> MDNSNGIHYIELTPNPIRFDAVSQLTNVFFDDSNKQIFAVRSGGATGVVVKGPGSPDDVVISFCMSDRGGAIRSIKFSPDNQILAVQRKENSVEFICFQGDQPLLQDIITHQVKTLIHGFVWVHNREVALISNTGVEVYTVVPEKRQVRSVKSLSIGIKWFAWCCDANVALLCTSEGNSLIPVLVKQKVITKLPKVDLGNPSRDVQESKVTLGQVYGVLAVLILQSNSTTGLMEVEVHLLNGPGLAPRKCHVLRLSLLGRFAINTVDNLIVVHHQASGTSLLFDISLPGEVINEITYHTPITPGRSIKPFGLKLPSLSPDGQILQCELYSTHWVLFQPNIVIDAKLGCMWFLNLCIEPLCQLISDRIRLTEFLLQRSNGKQMLLKVIGQLVDDQYKGTLLPVLETIFSRINKIYASWVQLELQNQTAQPSNVKTTTLKQSTPPIVLIEQLDMVQIFQRIARRPYTESILMLYLQSLNKFNIAAQEELSKMIISELISNRSFDTLRRLVSYSMLLESKSVACFLLSHSNVDTAISQVAIDMLGRIEAHEIIIEVMLGQGKVIDALRLAKNSMGLEKVPARKFLEAAHKTKDDLIFHSVYRFFQMRNLKLYETLSFPKAEQCTEFIQHYNNTFPADNPTRQPVS;> MAKLLQRVEITLRSFYIFNSTFGQVEGEEHKKVLFYHPNDIELNTKIKDVGLSEAIIRFTGTFTSEDDCQALHTQKTTQLFYQPEPGYWLVLVLNVPKEVRLKEGVEVADYRGAEISDRIYRAILRQCYQMFRFQNGCFSSCGSEEPNPDKRRELLCQKLLQFYDQHLTNLRDPAQCDIIDMLHSIQYLPLDKTLFLRAQNFGTLCETFPDIKESIMLYQEQVLCGGKLSPEDLHCVHSYV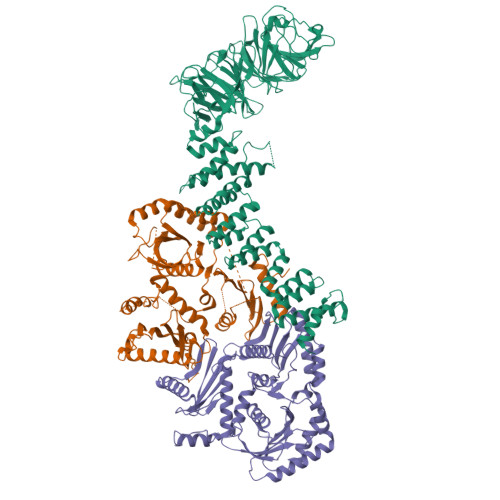VQHVLKVEASSSTIAVSPSLKRSISECQVGGFVRSRQKVAGDEHDAVNEEDHPMKVYVTLDKEAKPYYLLIYRALHITLCLFLNADQVAPKQDLYDDLHAYMAPQLTSLARDISSELTKEAVGAAGQDNSSGNSETAPKYLFINEQSLQHHTNFQRHLPQGLPRNVLSIIADLANGSGKAEMESAPAEEVQVKTTNDYWIVKRRCNYRQYYVILCNSKATLLDVTQEARRIFEQELTDDVFFDK;> HHHHHHHHHHENLYFQGGGSMEVEQTSVRSDTNSTCEYLDAEGDPESPNLYQEADPDQEAEQQNHSIISELRDGLGTMRDNSALSPEPGQENKGLAASVESLALSTSTSAKTEDSIGGGLEEEYDYQHDSLWQGQKKHIFILSEAGKPIFSLHGNEDKLATLFGVIQALVSFVQMGQDAITSIHAGGIKFAFMQRSSLILVAASRSNMSVQQLQLQLGDVYNQILSILTYSHMTKIFERRKNFDLRRLLSGSERLFYNLLANDSSSAKVSNNIFTFLTNSIRVFPLPTTIRSQITSAIQSNCSKIKNLVFAVLIANNKLIALVRMKKYSIHPADLRLIFNLVECSESFKSSENWSPICLPKFDMNGYLHAHVSYLADDCQACLLLLSVDRDAFFTLAEAKAKITEKLRKSHCLEAINEELQQPFNAKLYQQVVGIPELRHFLYKPKSTAQLLCPMLRHPYKSLTELERLEAIYCDLLHRIHNSSRPLKLIYEMKEREVVLAWATGTYELYAIFEPVVDKATVIKYVDKLIKWIEKEYDVYFIRNHATF> ELPTDCGGPFELWEPNTTFSSTNFPNSYPNLAFCVWILNAQKGKNIQLHFQEFDLENINDVVEIRDGEEADSLLLAVYTGPGPVKDVFSTTNRMTVLLITNDVLARGGFKANFTTGYHLGIPEPCKADHFQCKNGECVPLVNLCDGHLHCEDGSDEADCVRFFNGTTNNNGLVRFRIQSIWHTACAENWTTQISNDVCQLLGLGSGNSS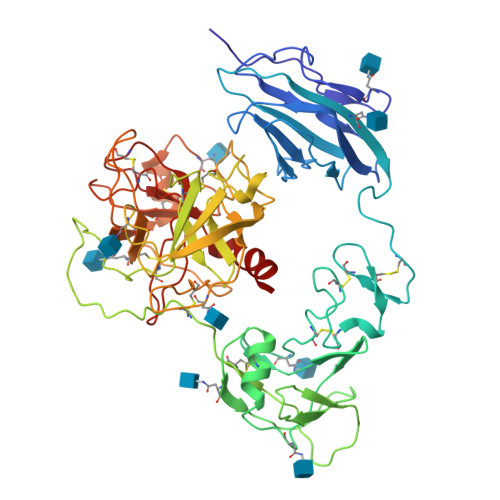KPIFPTDGGPFVKLNTAPDGHLILTPSQQCLQDSLIRLQCNHKSCGKKLAAQDITPKIVGGSNAKEGAWPWVVGLYYGGRLLCGASLVSSDWLVSAAHCVYGRNLEPSKWTAILGLHMKSNLTSPQTVPRLIDEIVINPHYNRRRKDNDIAMMHLEFKVNYTDYIQPICLPEENQVFPPGRNCSIAGWGTVVYQGTTANILQEADVPLLSNERCQQQMPEYNITENMICAGYEEGGIDSCQGDSGGPLMCQENNRWFLAGVTSFGYKCALPNRPGVYARVSRFTEWIQSFLH> MFDYETLRFIWWLLIGVILVVFMISDGFDMGIGCLLPLVARNDDERRIVINSVGAHWEGNQVWLILAGGALFAAWPRVYAAAFSGFYVAMILVLCSLFFRPLAFDYRGKIADARWRKMWDAGLVIGSLVPPVVFGIAFGNLLLGVPFAFTPQLRVEYLGSFWQLLTPFPLLCGLLSLGMVILQGGVWLQLKTVGVIHLRSQLATKRAALLVMLCFLLAGYWLWVGIDGFVLLAQDANGPSNPLMKLVAVLPGAWMNNFVESPVLWIFPLLGFFCPLLTVMAIYRGRPGWGFLMASLMQFGVIFTAGITLFPFVMPSSVSPISSLTLWDSTSSQLTLSIMLVIVLIFLPIVLLYTLWSYYKMWGRMTTETLRRNENELY;> MWDVIDLSRWQFALTALYHFLFVPLTLGLIFLLAIMETIYVVTGKTIYR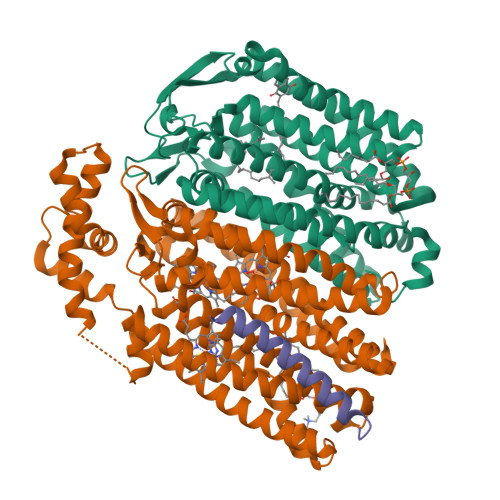DMTRFWGKLFGINFALGVATGLTMEFQFGTNWSFYSNYVGDIFGAPLAMEALMAFFLESTFVGLFFFGWQRLNKYQHLLVTWLVAFGSNLSALWILNANGWMQYPTGAHFDIDTLRMEMTSFSELVFNPVSQVKFVHTVMAGYVTGAMFIMAISAWYLLRGRERNVALRSFAIGSVFGTLAIIGTLQLGDSSAYEVAQVQPVKLAAMEGEWQTEPAPAPFHVVAWPEQDQERNAFALKIPALLGILATHSLDKPVPGLKNLMAETYPRLQRGRMAWLLMQEISQGNREPHVLQAFRGLEGDLGYGMLLSRYAPDMNHVTAAQYQAAMRGAIPQVAPVFWSFRIMVGCGSLLLLVMLIALVQTLRGKIDQHRWVLKMALWSLPLPWIAIEAGWFMTEFGRQPWAIQDILPTYSAHSALTTGQLAFSLIMIVGLYTLFLIAEVYLMQKYARLGPSAMQSEQPTQQQG;> MWYLLWFVGILLMCSLSTLVLVWLDPRLKSIEGRGTSGSSGSGSGGSGSGGGGWSHPQFEK>[16x]MKNLDINTFDNIEDIPLGSSEQDPYDFFTLSDRNVMNSDMKKNIVQWNSRYSYNQLKNKDSLIMFLVEIFRSLFVSNCIDKNIDNVLLSIEEMFIDHYYNPQHSRLKYLIDDVGIFFTKLPITKAFHTYNKKYRITKRLYAPPTFNEVRHILNLAQILSLEEGLDLLTFDADETLYPDGHDFNDEVLASYISCLLKKMNIAIVTAASYNNDAEKYQKRLENLLKYFSKHNIKDGSYKNFYVMGGESNYLFKCNEEATLYSVPENEWRHYKKFVDYDTVQEILNISEKCLEKVIKDFGLCAQIQRKEKSIGLVPNKIPSLNIKNEQKNYMIKYEVLEEAVIRIKKEIIKNKITAPYCAFNGGQDLWVDVGNKAEGLLILQKLLKIQKKKCCHIGDQFLHSGNDFPTRFCSLTLWVSNPQETKACLKSIMHLNIKSFIPEVLYENQ

Maintaining the optimal nucleotide balance required for normal cell proliferation is controlled by 5′-nucleotidases amongst other processes. These enzymes catalyze the dephosphorylation of ribo- and deoxyribonucleoside monophosphates to their corresponding nucleosides, and also exhibit, in certain cases phosphotransferase activity. All structures adopt a tetrameric assembly displaying a cross-like shape, in agreement with the quaternary solution structure. Each subunit consists of four domains: an “N-Terminal Regulatory Domain” (NTRD, M1 to K59), an “OD” (D60 to T143), a HAD-like Catalytic Domain (CD, F144 to K270 and K371 to Q444) and a C2 cap domain13 (K271 to N370).

Finally, the NTRD is mainly composed of a random coil, exempting helices α1 and α2, both situated at interface 1 between α and β subunits (or between γ and δ subunits) in the apo conformation (PfISN1-Apo). However, the cavity created by the interaction between the two subunits at interface 1 can accommodate only one NTRD at a time, forcing the second NTRD to localize elsewhere. No extra density is observed for this latter NTRD up to residue 59, thereby suggesting it being highly flexible. When superimposing subunits with and without NTRD, the overall structures are very similar (RMSD 0.4 Å). Analyses of PfISN1-Apo SAXS data confirm the high flexibility of two NTRDs, and SAXS restrained modelling indicates that unstructured NTRDs may be located at interface 2. In PfISN1-Apo, helix α8 (residues 171–175) carrying one of the catalytic aspartates, occupies the binding site of the phosphate moiety and Mg2+. In this conformation, E173 (Motif 1) interacts with H398 (Motif IV) while D178 and D394 are exposed to the solvent. NTRDs in conformation 1 are entirely structured as observed in α and γ subunits of PfISN1-Apo and PfISN1-ATP, being stabilized by several hydrogen bonds and two salt bridges (K41-D394 and D60-R406). In conformation 2, NTRDs are not visible in the electron density from residues 1–59 as in the case for β- and δ subunits of PfISN1-Apo and PfISN1-ATP, but floating in the solvent as suggested by SAXS data.> MADGFFKQLTLPSGQVVTVSEGRGEPASTGSYDVRLYSGANPQFPLDQFI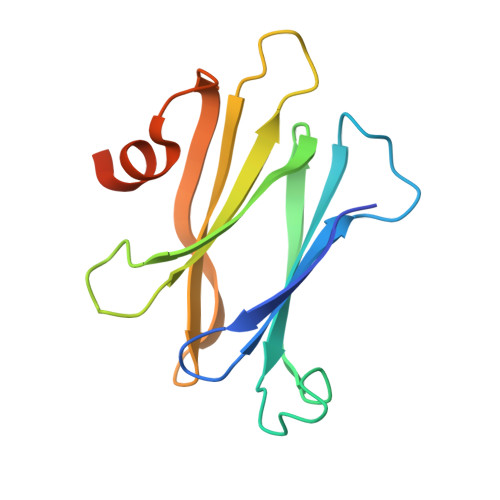DGKVLPRDGSIKELKLLDLNGDKQPELIVVVESAGSGSYLSADAFTLNPQEGLDSFNHVEGLAPNEDVIQALKTPRDLEHHHHHH>[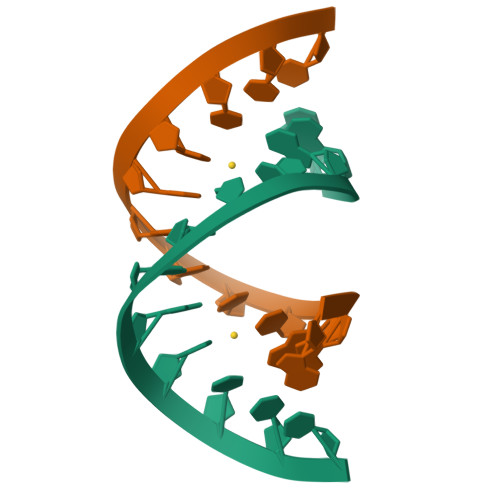4x]GGACUCGACUCC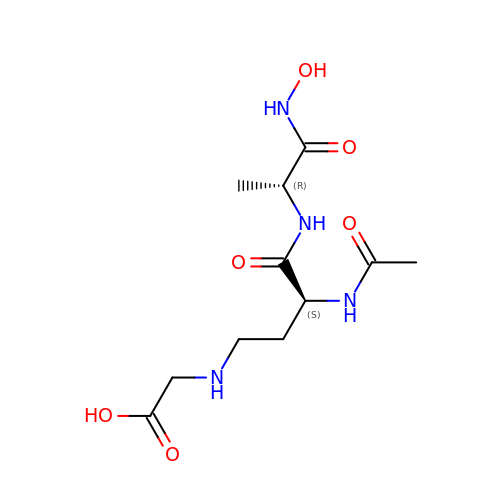2-[[(3S)-3-acetamido-4-[[(2R)-1-(oxidanylamino)-1-oxidanylidene-propan-2-yl]amino]-4-oxidanylidene-butyl]amino]ethanoic acid | C11 H20 N4 O6 | SPJUSNPGUPFCMZ-SVRRBLITSA-N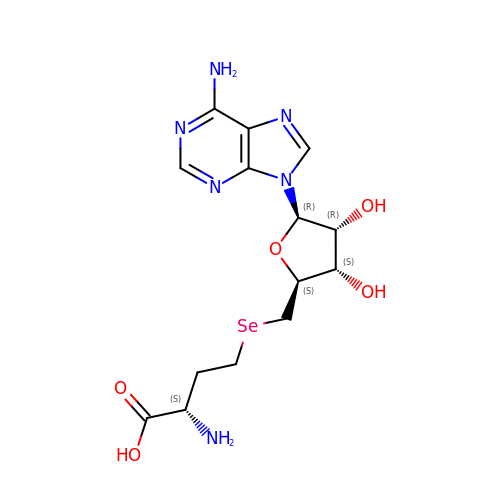S-ADENOSYL-L-HOMOSELENOCYSTEINE | C14 H20 N6 O5 Se | UVSMMLABJBJNGH-WFMPWKQPSA-N>[4x]RDSG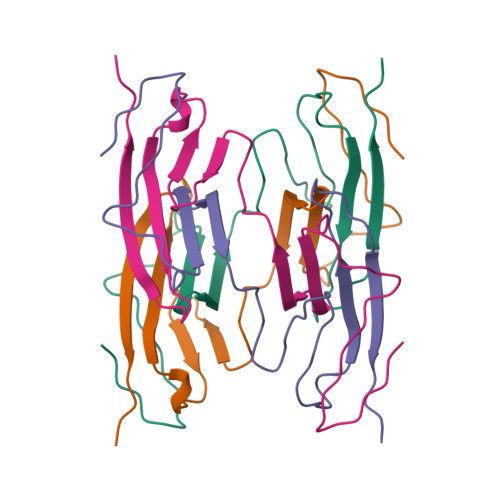TVWGALGHGINLNIPNFQMTDDIDEVRWERGSTLVAEFKRKPFLKSGAFEILANGDLKIKNLTRDDSGTYNVTVYSTNGTRILDKALDLRILE> RYSVYWKGNRRSIAEGGSSGTINVLDHGAKGDGTSDDTKAFEDAWQVACKVAASTLLVPSGSTFLVGPVSFLGKECKEKIVFQLEG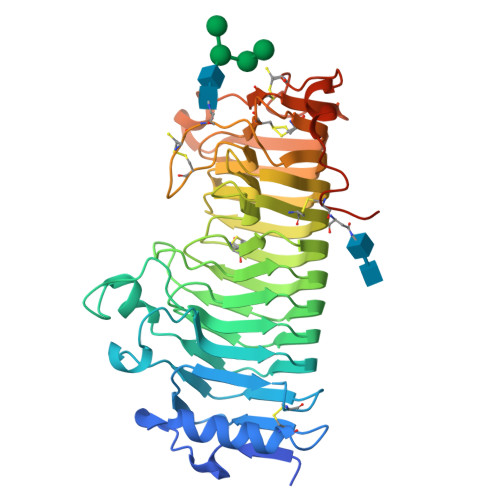KIIAPTSASAWGSGLLQWIEFKALQGITIKGKGIIDGRGSVWWNDMMGTKMPRTKPTALRFYGSNGVTVSGITIQNSPQTHLKFDNCISIQVSDFTTSSPGDSPNTDGIHLQNSQDAVIYRSTLACGDDCISIQTGCSNINIHDVDCGPGHGISIGGLGKDNTKACVSNITVRDVTMHETTNGVRIKSWQGGSGSVKQVMFSNIQVSNVANPIIIDQYYCDGGGCHNETSAVAVSNINYINIKGTYTKEPVRFACSDSLPCTGISLSTIELKPATGKASSLDPFCWKAHGELKTKTLPPIQCLKTEKSPEAASRSNNDACFLEQKLISEEDLNSAVDHHHHHH> MSEMTPREIVSELDKHIIGQDNAKRSV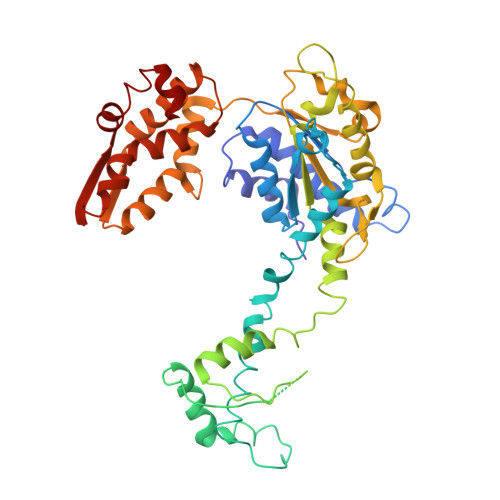AIALRNRWRRMQLNEELRHEVTPKNILMIGPTGVGKTEIARRLAKLANAPFIKVEATKFTEVGYVGKEVDSIIRDLTDAAVKMVRVQAIEKNRYRAEELAEERILDVLIPPAKNNWGQTEQQQEPSAARQAFRKKLREGQLDDKEIEIDLAAAPMGVEIMAPPGMEEMTSQLQSMFQNLGGQKQKARKLKIKDAMKLLIEEEAAKLVNPEELKQDAIDAVEQHGIVFIDEIDKICKRGESSGPDVSREGVQRDLLPLVEGCTVSTKHGMVKTDHILFIASGAFQIAKPSDLIPELQGRLPIRVELQALTTSDFERILTEPNASITVQYKALMATEGVNIEFTDSGIKRIAEAAWQVNESTENIGARRLHTVLERLMEEISYDASDLSGQNITIDADYVSKHLDALVADEDLSRFIL> MENTENSVDSKSIKNLEPKIIHGSESMDSGISLDNSYKMDYPEMGLCIIINNKNFHKSTGMTSRSGTDVDAANLRETFRNLKYEVRNKNDLTREEIVELMRDVSKEDHSKRSSFVCVLLSHGEEGIIFGTNGPVDLKKITNFFRGDRCRSLTGKPKLFIIQACRGTELDCGIETDSGVDDDMACHKIPVDADFL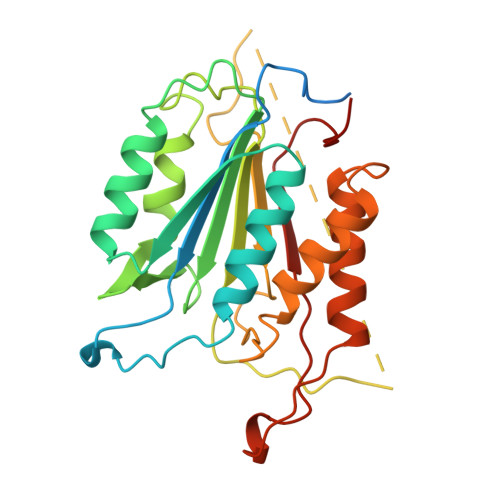YAYSTAPGYYSWRNSKDGSWFIQSLCAMLKQYADKLEFMHILTRVNRKVATEFESFSFDATFHAKKQIPCIVSMLTKELYFYH>MGADPVYGLPGFGDHEGRTPFKRLQVSDIVAIRTPVRITPDRKAFWRKYMSYESPFHLNDAVAIVTGAAAGIGRAIAGTFAKAGASVVVTDLKSEGAEAVAAAIRQAGGKAIGLECNVTDEQHREAVIKAALDQFGKITVLVNNAGGGGPKPFDMPMSDFEWAFKLNLFSLFRLSQLAAPHMQKAGGGAILNISSMAGENTNVRMASYGSSKAAVNHLTRNIAFDVGPMGIRVNAIAPGAMKTDALATVLTPEIERAMLKHTPLGRLGEAQDIANAALFLCSPAAAWISGQV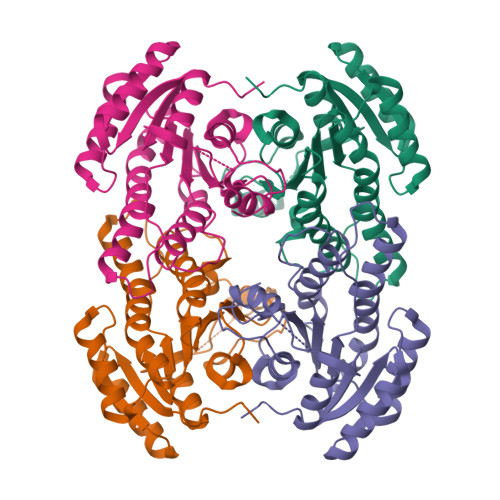LTVSGGGVQELD[4x]A hallmark of all motile M. xanthus cells is the accumulation of MglA-GTP at the leading pole where it activates motility, while MglA-GDP is found diffusely in the cytosol. This localization pattern arises due to the GAP activity of MglB, which is located at the lagging pole where it inactivates MglA-GTP and depletes it from this pole. The ability of MglA to hydrolyze GTP is essential for motility regulation. To gain insight into the structural landscape of M. xanthus MglA, we determined the crystal structures of MglA in different nucleotide states, which uncovered that MglA can adopt three conformations: inactive MglA-GDP, active MglA-GTPγS, whose structure had not been determined before, and an unusual conformation combining inactive and active features.

Next, we determined the crystal structure of the M. xanthus MglA-GTPγS/MglB complex. The complex contains a symmetrical MglB dimer and one MglA-GTPγS molecule, as previously observed for T. thermophilus MglA-MglB complexes. As in unbound MglB, the C-terminii of MglB are disordered in the MglA-MglB complex. Both MglB monomers interact through their helix 2 with switch 1 and switch 2 of MglA, which display active conformations, with one monomer establishing additional contacts outside the switch regions. The MglB dimer does not insert any element in the nucleotide-binding site and does not interact with GTPγS directly. Overlay of unbound MglA-GTPγS shows that one MglB monomer would clash with the arginine finger loop, a conflict that is resolved by a large lasso movement of switch 1 (11 Å at Arg53). This rearrangement positions the arginine finger near the active site, which it could reach through side chain rotation, and it completes the canonical coordination of Mg2+ by the conserved switch 1 threonine (Thr 54). Thus, MglB recognizes the active conformations of the switch regions and contributes to catalysis by reorganizing the arginine finger loop through steric conflict. The organization of the MglA-MglB complex is surprisingly similar to that of the complex of the Rab GTPase Ypt1 with the TRAPP complex, a yeast RabGEF whose central subunits have roadblock folds. The slow spontaneous GDP/GTP exchange of MglA was not increased by MglB, indicating that MglB does not function as a GEF under these conditions.

> MSFINYSSREINCKIVYYGPGLCGKTTNLQYIYNKTAAETKGKLISLSTETDRTLFFDFLPLSLGEIRGFKTRFHLYTVPGQVFYDASRKLILKGVDGVVFVADSQIERMEANMESLENLRINLAEQGYDLNKIPYVIQYNKRDLPNAVTVEEMRKALNHRNIPEYQAVAPTGVGVFDTLKAVAKLVLTELKKGGHHHHHH;>GMGTQLVMYEEEFTKINAVCDRLTKDANAKVVFLVDKNGQLISSAGQTQNIDTTSLASLTAGNVAAMGGLAKLIGENEFPNQFHEGAKDSLYMTIVGSRVVLVVIFDNRTSLGLVRLRIKKASDELTKIFESLVKKTDSPGAGSPFAEISDDDIDNLFSE[2x]> MDAELAEVRALQAEIAALRRACEDPPAPWEEKSRVQKSFQAIHQFNLEGWKSSKDLKNQLGHLESELSFLSTLTGINIRNHSKQTEDLTSTEMTEKSIRKVLQRHRLSGNCHMVTFQLEFQILEIQNKERLSSAVTDLNIIMEPTECSELSEFVSRAEERKDLFMFFRSLHFFVEWFEYRKRTFKHLKEKYPDAVYLSEGPSSCSMGIRSASRPGFELVIVWRIQIDEDGKVFPKLDLLTKVPQRALELDKNRAIETAPLSFRTLVGLLGIEAALE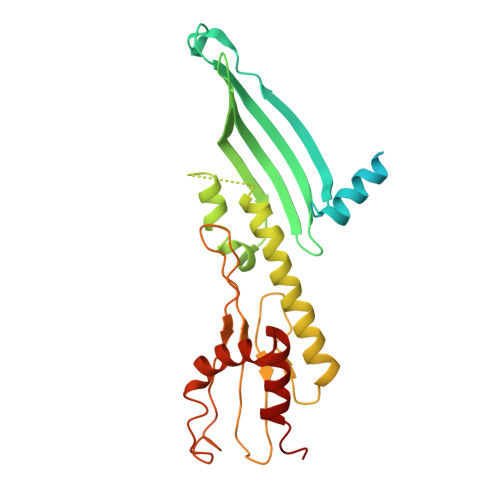SLIKSLCAEENN> MEAVLNELVSVEDLLKFEKKFQSEKAAGSVSKSEQFEYAWCLVRSKYNDDIRKGIVLLEELLPKGSKEEQRDYVFYLAVGNYRLKEYEKALKYVRGLLQTEPQNNQAKELERLIDKAMKKDGLLEVLFQ

A tetratricopeptide repeat (TPR) motif containing mitochondrial outer membrane protein, mitochondrial fission protein 1 (Fis1), mediates mitochondrial fission by recruiting large cytosolic GTPase, Drp1, to the mitochondrial outer membrane. The cytosolic domain of Fis1 is composed of 6 tight α-helices with two anti-parallel TPR motifs forming a concave hydrophobic surface. Fis1 interaction with Drp1 occurs during cellular stress, but not under physiological conditions, suggesting that cellular signals during stress activate Fis1. Human Fis1 protein contains a single cysteine, Cys41, in the entire protein.

To explore this possibility further, we crystallized and determined the X-ray structures of the WT and three phosphorylation mimic-mutants of Fis1: Thr34Asp Fis1, Thr34Glu Fis1 and Tyr38Glu Fis1. Each of these mutants was previously shown to be sufficient to increase Drp1 recruitment to mitochondria and subsequent mitochondrial fission in cell-based studies. Consistently, we observed that the first 30 residues including the α1 helix were missing from the structure providing strong evidence that the α1 helix undergoes significant conformational change and is potentially disordered in the phosphorylated forms, whereas it was intact in the WT. We crystallized the phosphorylation-mimic mutants, Thr34Asp, Thr34Glu and Tyr38Glu Fis1, and we observed that in all the cases, these mutants crystallized as covalent dimers mediated by Cys41 disulfide bridge between two Fis1 protomers. As Thr34Asp, Thr34Glu and Tyr38Glu Fis1 have a greater propensity for a conformationally altered N-terminus and hence have more exposed Cys41, they crystallized as covalent dimers. Upon closer examination of the crystal structures, we observed that the concave hydrophobic surface in the covalent dimers of all the phosphorylation-mimic mutants was exposed. Our crystal structure not only shows the absence of α1 helix but also shows that there is no space for structured α1 helix in the covalent dimer as this space is occupied by α2 helix of another monomer. Here we showed that Cys41 is also oxidizable and mediates Fis1 covalent dimerization through disulfide linkage. This oxidation-induced Fis1 dimerization was obvious in the crystal structures of Thr34Asp, Thr34Glu and Tyr38Glu Fis1, where we saw a clear electron density for the disulfide linkage.>[4x]GMLEFTKRSLMNKYNINERVLELYERALNDVEKEFKYYDEIREYNQLKVLKAFQEERISESHFTNSSGYGYNDIGRDSLDRVYANIFNTESAFVRPHFVNGTHAIGAALFGNLRPNDTMMSICGMPYDTLHDIIGMDDSKKVGSLREYGVKYKMVDLKDGKVDINTVKEELKKDD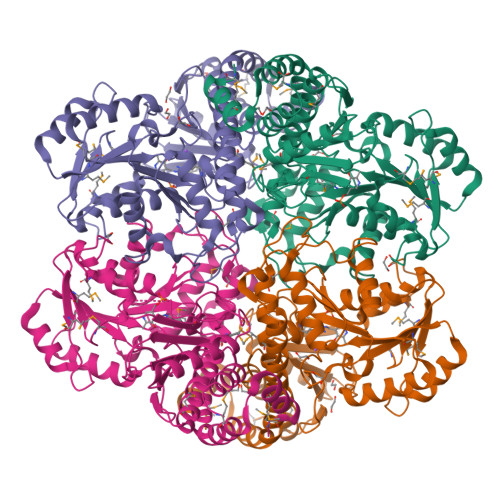SIKLIHIQRSTGYGWRKSLRIAEIAEIIKSIREVNENVIVFVDNCYGEFVEEKEPTDVGADIIAGSLIKNIGGGIATTGGYIAGKEEYVTQATFRVTVPGIGGECGSTFGVMRSLYEGLFMAPHVTIEAVKGAVFCARIMELAGFDVLPKYNDKRTDIIQAIKFNDEKKLIDFIKGIQTASPVDSFVQCEAWDMPGYEDKVIMAAGTFVQGASIELSADAPIREPYIGYLQGGLTFDHAKLGVLIALSKLIM The microscopic openings across the walls of many capillaries contain a protein mesh that is formed by the extracellular domain (ECD) of plasmalemma vesicle-associated protein (PLVAP). Current evidence suggests that a single transmembrane protein, plasmalemma vesicle-associated protein (PLVAP or PV1), constitutes the diaphragm’s sole structural protein. PLVAP is a type II transmembrane protein of ~60 kDa with an ~390-amino acid C-terminal extracellular domain (ECD), a single transmembrane domain, and a 26-amino acid N-terminal cytoplasmic domain. The three-dimensional structure of PLVAP CC1 presented here shows that it forms a parallel disulfide-bonded dimeric coiled coil.

PLVAP CC1 is 89 amino acids in length and contains five cysteines. PLVAP CC1 contains five cysteines and one methionine, and previous studies have demonstrated that SAD from sulfur-containing residues—sulfur SAD—can be used for experimental phasing and structure determination. For this experiment, we first screened additional crystallization conditions and obtained PLVAP CC1 crystals in the P212121 space group with unit-cell parameters 35.6 Å, 86.2 Å, and 181.6 Å, referred to hereafter as crystal form I. We then collected data at a wavelength of 1.77 Å, using a low-noise and fast readout EIGER X detector, with an exposure time of 0.015 s per 0.2° oscillation. The data collection encompassed a total rotation of 1,800° while continuously advancing the crystal 300 μm. Constraints related to the detector-to-crystal distance and the long wavelength of the X-ray beam limited the resolution of the sulfur SAD data to 2.4 Å. The structure of PLVAP CC1, determined from crystal form I by sulfur SAD, reveals a parallel dimer with five symmetric interchain disulfide bonds (SS-1 by Cys142, SS-2 by Cys153, SS-3 by Cys178, SS-4 by Cys199, and SS-5 by Cys224). The five disulfide bonds were confirmed in the anomalous difference map. The electron density for residues 141 to 145 of crystal form II chain B was not visible. Structure-based analysis by the Socket2 algorithm for both crystal forms shows that most of the PLVAP CC1 dimer exhibits a classical coiled-coil configuration characterized by heptad repeats (abcdefg in Fig. 6A). Among PLVAP CC1 dimers, the average rmsds are 1.15 Å for crystal form I chain A + B vs. chain C + D, 0.89 Å for crystal form I chain A + B vs. crystal form II chain A + B, and 0.84 Å for crystal form I chain C + D vs. crystal form II chain A + B. Conformational differences are greatest at the N terminus.

>GPGTSRQCQEQLKEVNKTCEALLFKLGEKVKTLEMEVAKEKAVCSKDKESLLAGKRQTEEQLEACGKARERQQQEQQVTEENLRKVQSLCIPLDQ[4x]>MHHHHHHHHPDLGTGSENLYFQGLNSTAQGQLKSIIERVERLEVEKAEIMEQIKEVYAEAKGNGFDVKVLKKVVRIRKQDRAKRQEEDAILDLYLSAIGEI[6x]

GapR is an essential NAP in Caulobacter crescentus involved in DNA replication, chromosome segregation and cell division. In this paper we present three crystal structures of GapR from C. crescentus, crystallised in the presence of double-stranded DNA with a sequence from the origin of chromosome replication. In all three structures, GapR adopts the same overall tetramer ring form as seen by Guo et al., albeit with small but important increases in the diameter of the central channel. DNA could not be visualized in any of our three structures, but DNA could be detected in gel electrophoresis, indicating that DNA is present in the crystals.

For this, we used both full length GapR and GapRΔ1-11 (a construct in which we removed the first eleven residues, that were predicted to be disordered) and a 19-bp dsDNA oligomer with a sequence from the C. crescentus origin of replication, which GapR binds with a nanomolar dissociation constant. We were also able to solve the structure of GapRΔ1-11 from crystals of space group P4322. Diffraction from these crystals also showed high anisotropy, with resolution limits between 3.3 Å and 3.8 Å. Following ellipsoidal truncation and anisotropic correction using the Diffraction Anisotropy Server10 the structure was refined to an Rfree of 0.322. There are six monomers in the asymmetric unit, arranged as a tetramer and a dimer. The tetramer could be overlaid onto the I4132 tetramer with an rmsd of 1.9 Å. Crystallographic symmetry again showed that the dimer of the asymmetric unit paired with symmetry-related molecules to form tetramers. Furthermore, in the I4132 and P4322 structures, a 19 bp DNA oligio would have to adopt substantial bends to thread through the central channel of adjacent tetramers, because channels formed by adjacent GapR tetramers do not line up. The main difference between GapR in the three crystal forms arises from slight changes in the orientation of helix three, which results in minor variations in the size of the central channel.>MSDIFDEAASFRSYQSKLGRDGRASAATATLTTKIRIFVPATNSPELRWELTLFALDVIRSPSAAESMKIGAAFTLISMYSERPGALIRSLLNDPDIEAVIIDVGSMLNGIPVMERRGDKAQEEMEGLMRILKTARESSKGKTPFVDSRAYGLRITDMSTLVSAVITIEAQIWILIAKAVTAPDTAEESETRRWAKYVQQKRVNPFFALTQQWLTEMRNLLSQSLSVRKFMVEILMEVKKGGSAKGRAVEIISDIGNYVEETGMAGFFATIRFGLETRYPALALNEFQSDLNTIKGLMLLYREIGPRAPYMVLLEESIQTKFAPGGYPLLWSFAMGVATTIDRSMGALNINRGYLEPMYFRLGQKSARHHAGGIDQNMANKLGLNSDQVAELAAAVQETSVGRQDNNMQAREAKFAAGGVLVGGGEQDIDEEEEPIEHSGRQSVTFKREMSMSSLADSVPSSSVSTSGGTRLTNSLLNLRSRLAAKAIKESTAQSSSERNPPNNRPQADSG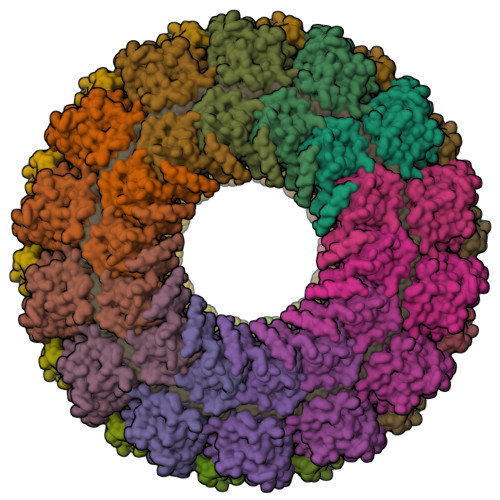RKDDQEPKPAQNDLDFVRADV[28x]>QADFEHAISDLEAHNQAKIGVALVSENGNLIQGYRANERFAMCSTFKLPLAALVLSRIDAGEENPERKLHYDSAFLEEYAPAAKRYVATGYMTVTEAIQSALQLSDNAAANLLLKEVGGPPLLTKYFRSLGDKVSRLDRIEPTLNTNTPGDERDTTTPMSMAQTVSKLIFGDTLTYKSKGQLRRLLIGNQTGDKTIRAGLPDSWVTGDKTGSCANGGRNDVAFFITTAGKKYVLSVYTNAPELQGEERA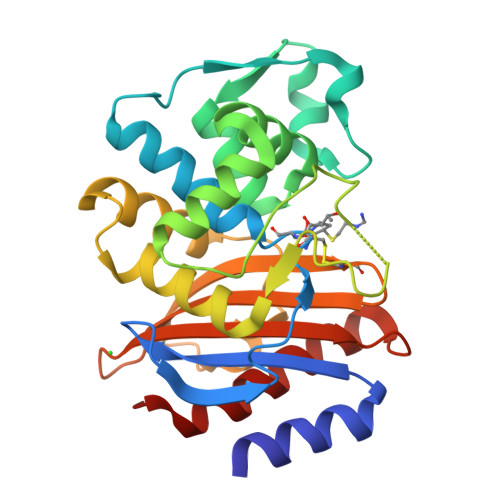LLIASVAKLARQYVVH[4x]> 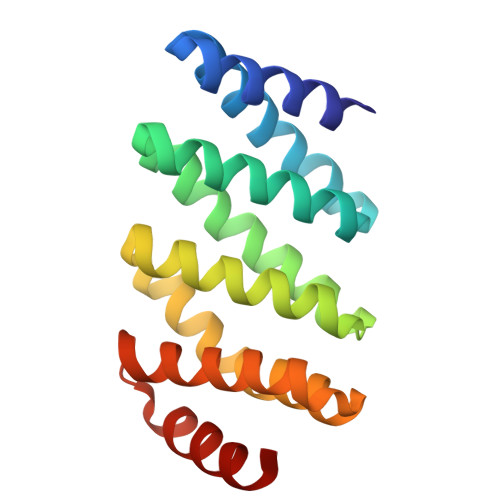SMLEEIERLVLSGLLTGDKELLKKASELLKEEMEKLLEEGDLDALKKALQLAVNVADHNGDKELLAHAAEVIKRALDLALEAKDLQSAKYLASLALWIAKRAGDKELYAYLEEKIKKIIELAEEAGDRESLKILILLGIFIARDAGSEEVKAFVAEQLERLL5'-O-(ethylcarbamoyl)guanosine 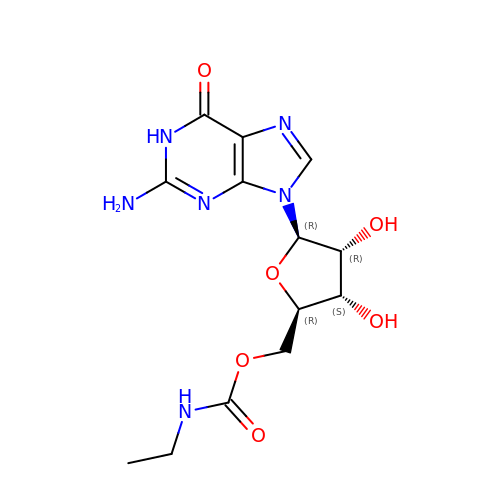| C13 H18 N6 O6 | UQGAPQHFXCJSGR-IOSLPCCCSA-N> MTSFQ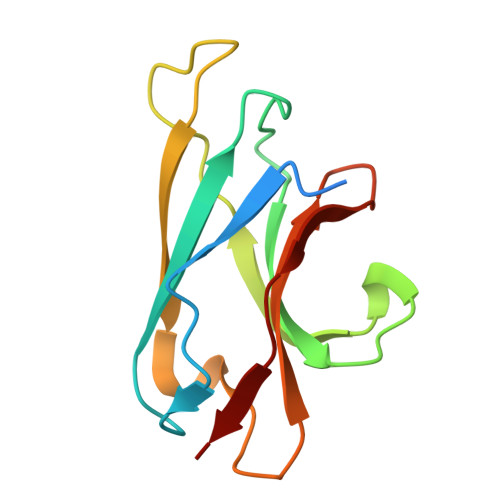EVPLQTSNFAHVIFQNVAKSYLPNAHLECHYTLTPYIHPHPKDWVGIFKVGWSTARDYYTFLWSPMPEHYVEGSTVNCVLAFQGYYLPNDDGEFYQFCYVTHKGEIRGASTPFQFR(8~{S})-6-[2-(2,3-dihydroindol-1-yl)-2-oxidanylidene-ethyl]-4-(4-methylphenyl)-2-oxidanylidene-8-propyl-1,5,7,8-tetrahydro-1,6-naphthyridine-3-carbonitrile | 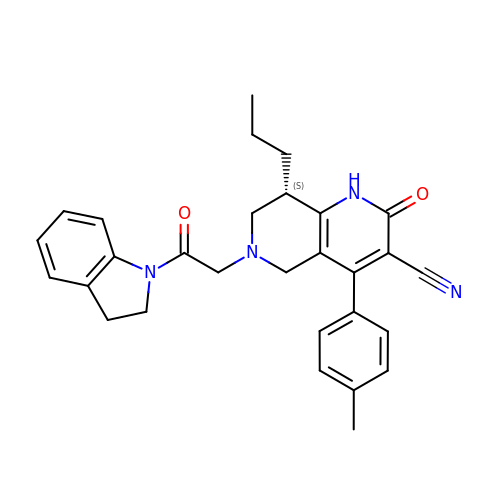C29 H30 N4 O2 | TVUOEVCKUGISBU-QFIPXVFZSA-N5H-PYRAZOLO(1,2-A)(1,2,4)TRIAZOL-4-IUM, 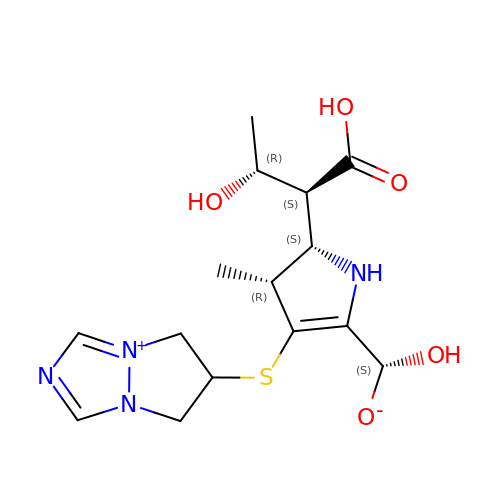6-((2-CARBOXY-6-(1-HYDROXYETHYL)-4-METHYL-7-OXO-1-AZABICYCLO(3.2.0)HEPT-2-EN-3-YL)THIO)-6,7-DIHYDRO-, HYDROXIDE, INNER SALT, (4R-(4ALPHA,5BETA,6BETA(R*)))- | C15 H22 N4 O5 S | GJACIOMQYIQIKX-FGOODDOWSA-N>GIDFPTMLKIKLEKTTFENAKAECSLVFIINKDFSHAWVKNKELLETFKYEGEGVFLDQENKILYAGVKEDDVHLLRESACLAVRTLKKLAFKSVKVGVYTCGAHSKDNALLENLKALFLGLKLGLYEYDTFKSNKKESVLKEAIVALELHKPCEKTCANSLEKSAKEALKYAEIMTESLNIVKDLVNTPPMIGTPVYMAEVAQKVAKENHLEIHVHDEKFLEEKKMNAFLAVNKASLSVNPPRLIHLVYKPKKAKKKIALVGKGLTYDCGGL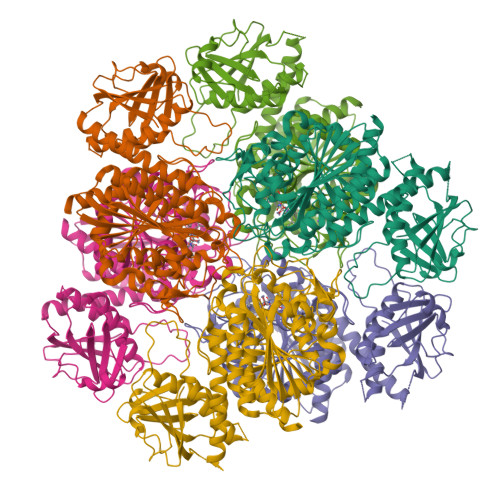SLKPADYMVTMKADKGGGSAVIGLLNALAKLGVEAEVHGIIGATENMIGPAAYKPDDILISKEGKSIEVRNTDAEGRLVLADCLSYAQDLNPDVIVDFATLTGACVVGLGEFTSAIMGHNEELKNLFETSGLESGELLAKLPFNRHLKKLIESKIADVCNISSSRYGGAITAGLFLNEFIRDEFKDKWLHIDIAGPAYVEKEWDVNSFGASGAGVRACTAFVEELLKKA[6x]(4~{S})-5-(3-chloranyl-2-fluoranyl-phenyl)-4-(4-chloranyl-2-methyl-phenyl)-3-propan-2-yl-1,4-dihydropyrrolo[3,4-c]pyrazol-6-one | C21 H18 Cl2 F N3 O 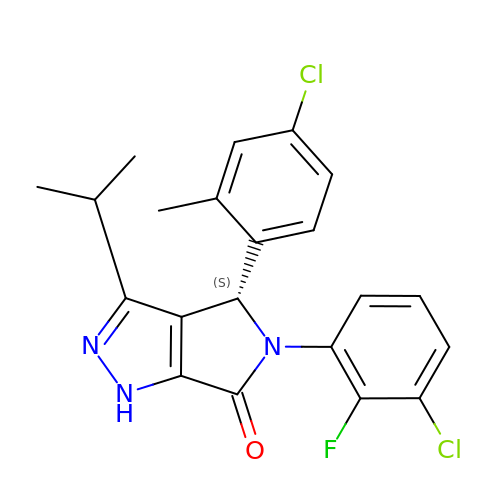| YQYGNXBWYDOKTG-FQEVSTJZSA-N>GSVQEAQANTESEKRRLDSVITHMSDGIIATDRRGRIRIVNDMALKMLGMAKEDIIGYYMLSVLSLEDEFKLEEI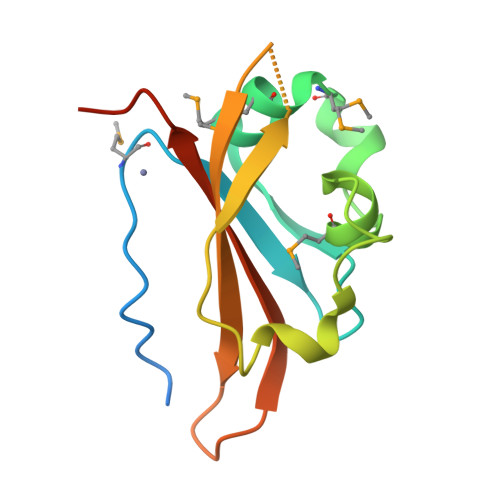QENNDSFLLDLNEEEGLIARVNFSTIVQETGFVTGYIAVLHDVTEQQQVERER[2x]>MHHHHHHSIKQNCLIKIINIPQGTLKAE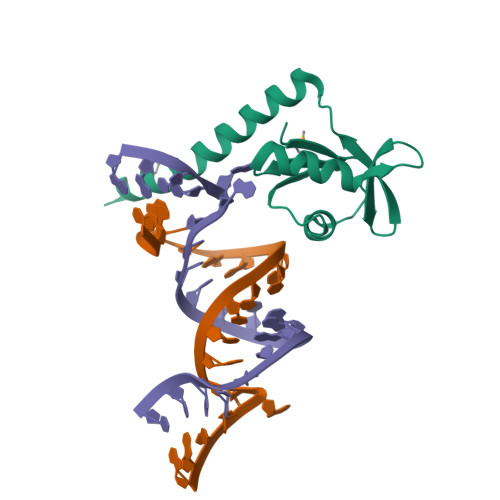VVLAVRHLGYEFYCDYIDGQAMIRFQNSDEQRLAIQKLLNHNNNKLQIEIRGQICDVISTIPEDEEKNYWNYIKFKKNEFRKFFFMKKQQKKQNITQNYNK[2x]> MSVHIEAKQGEIAESILLPGDPLRAKYIAETFLEDVTCYNNVRGMLGFTGTYKGKRVSVQGTGMGVPSISIYVNELIQSYGVKNLIRVGTCGAIQKDVKVRDVIIAMTACTDSNMNRLTFPGFDFAPAANFDLLKKAYDAGTEKGLHVRVGNVLTADVFYRESMDMVK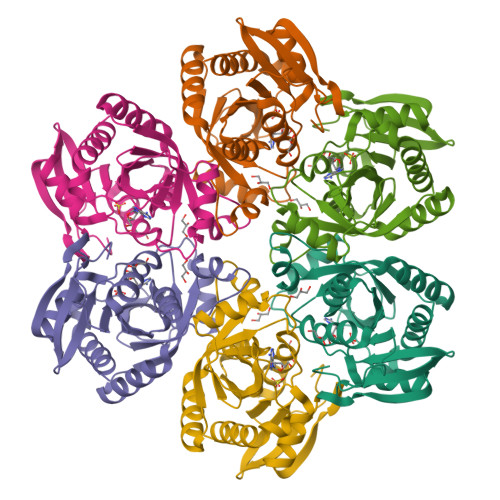KLGDYGVLAVEMETTALYTLAAKYGVNALSVLTVSNHIFTGEETTSEERQTTFNEMIEIALDAAIQQ>[2x]MLNVLMLGVGQCGNRILDAVNRQAFGGSRLAKYYSKQRFPSRVETIAINTAINDLKELKFTAAKDRLHVPNLHGVGANRSKGKQGFWENQEMILEEIEKRGDFDLIFVMTSVSGGTGSSFSPLMIHELKKRYKNATIVPIAVLPFREEGTIYLQNAAFCLREMIEVEADGMILVDNQYLKRFSGDIASAY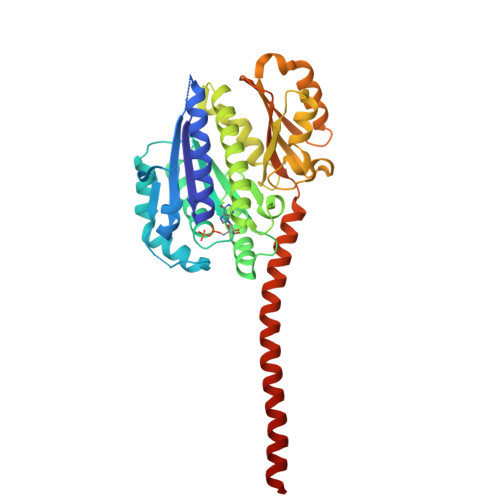DRINTMVAQRLLFLIEALDSEMLSVTDLGDFKTVMNGGLRMGTLGYYQADKKSPSIRAAIKNSLREVGLLYPANVDAGEAGRAMIVIQGSREYLNVDEITKEIESLTETIGHVFKGIVIKKGEPRVLSVLSLERAPGLVELYEKAKWAIQEERERKDRARSELYEAFEQINDLEEIYHHHHHH> MHHHHHHSSGRENLYFQGYVRDFKAKVQYFRFWCQQLAMPQHIKITVTRKTLFEDSFQQIMSFSPQDLRRRLWVIFPGEEGLDYGGVAREWFFLLSHEVSNPMYCLFEYAGKDNYCLQINPASYINPDHLKYFRFIGRFIAMALFHGKFIDTGFSLPFYKRILNKPVGLKDLESIDPEFYNSLIWVKENNIEECDLEMYFSVDKEILGEIKSHDLKPNGGNILVTEENKEEYIRMVAEWRLSRGVEEQTQAFFEGFNEILPQQYLQYFDAKELEVLLCGMQEIDLNDW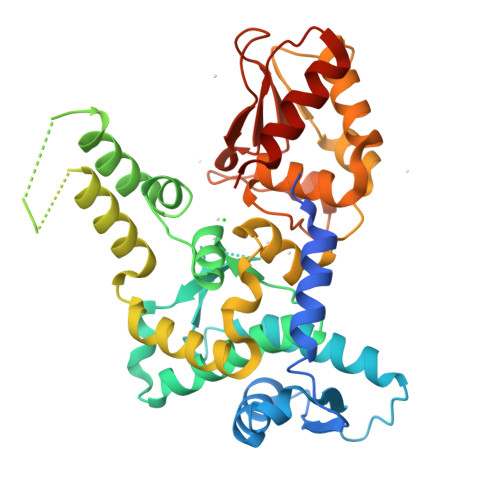QRHAIYRRYARTSKQIMWFWQFVKEIDNEKRMRLLQFVTGTCRLPVGGFADLMGSNGPQKFCIEKVGKENWLPRSHTCFNRLDLPPYKSYEQLKEKLLFAIEETEGFGQE>MSWQTYVDDHLMCDIDGHRLTAAAIIGHDGSVWAQSS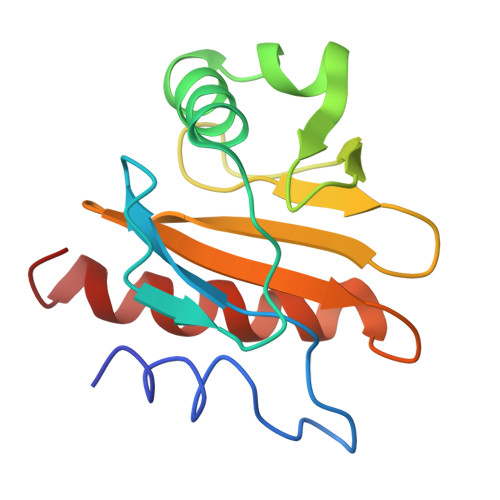SFPQFKSDEVAAVMKDFDEPGSLAPTGLHLGGTKYMVIQGEPGAVIRGKKGSGGITVKRTGQALIIGIYDEPLTPGQCNMIVERLGDYLLDQGL[2x]>[4x]MSQLVECVPNFSEGNNQEVIDAISQAISQTPGCVLLDVDAGPSTNRTVYTFVGQPECVVEGALSAARTASQLIDMRKHKGEHPRMGALDVCPFIPVRGVSMDECVLCAKAFGQRLAEELNVPVYLYGEAAQMPSRQTLPAIRAGEYEALPEKLKQAEWVPDFGPSSFVPSWGATVTGARKFLIAFNINLLSTKEQAHRIALNLREQGRGKDQPGRLKKVQGIGWYLEEKNLAQVSTNLLDFEVTALHTVYEEARREAQELNLPVVGSQLVGLVPLKALLDAAAFYCDKEKLFVLEEEHRIRLVVNRLGLDSLAPFDPKERIIEYLVPDSGPEQSLLDASLRAFVREVGARSAAPGGGSVAAAVAALGAALASMVGQMTYGRRQFDHLDSTMRRLIPPFHAASAQLTSLVDADARAFAACLGAIKLPKNTPEERDRRTCALQEGLRQAVAVPLKLAETVSQL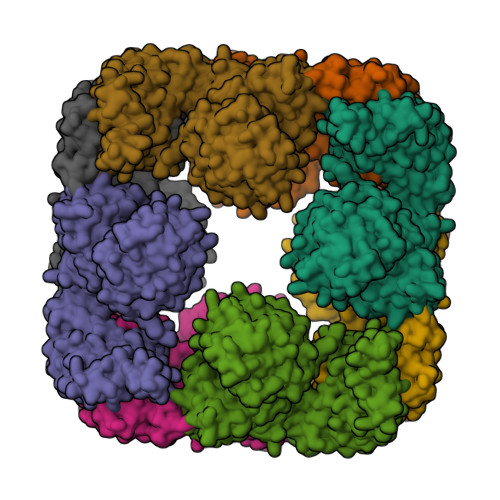WPALQELAQCGNLSCLSDLQVAAKALETGVFGAYFNVLINLKDMTDDVFKEKTRHRISSLLQEAKTQAALVLGSLEARKE The AS and TSL stack to form one continuous helical stack containing four GU base pairs, while the AC and DSL form another. The two helices are held in a roughly perpendicular orientation by interactions between the elements that are analogous to the D and T loops in tRNA.

We have determined the crystal structures of human mascRNA at 2.40 Å, human menRNA at 2.23 Å, and medaka mascRNA at 2.28 Å. Specifically, for mascRNA, these regions span nucleotides 1–7 and 51–57 for AS, 34–50 for TSL, 8–18 for DSL, and 19–33 for AC; for menRNA, they are 1–7 and 52–58 for AS, 35–51 for TSL, 8–17 for DSL, and 18–34 for AC. MascRNA and menRNA share ~70% sequence identity. The D loop of mascRNA is larger than that of menRNA, with the AC loop leaning more towards UUU. In contrast, the AC of menRNA is longer. Overall, they exhibit comparable conservation, suggesting a potential common evolutionary ancestor. Correspondingly, the tertiary structures of mascRNA and menRNA were well superimposed. In addition to the similarities in overall folding, the tertiary interactions that stabilize the L-shaped structure of menRNA resemble those of mascRNA. Apart from the elbow region, the base triplets G45-(cis Watson–Crick–Hoogsteen)-G8-(cis Watson–Crick)-C17 in menRNA are equivalent to the base triplets C16–G10–A44 in mascRNA, contributing to the resemblance in intramolecular interactions. However, the specific functions of menRNA are not fully understood, possibly due to its rapid degradation after the addition of a 3’ CCACCA sequence, making it challenging to detect using northern blot analysis.

>[2x]GGCGCUGGUGGUGGCACGUCCAGCACGGCUGGGCCGGGGUUCGAGUCCCCGCAGUGUU>[2x]MHHHHHHSSENLYFQGHMASMRIPEDVRKDIPLTNEVIYFDNTATSLTPKPVVEAMDEYYLKYRANVHRGVHRLSQMATHKYEESRKIVADFIGAKFEEIVFTKNTSESLNLVALGLGHIFKRGDKIVTTPYEHHSDLLPWQRLATKLGLKLEFIEGDDEGNLDLSDAEKKIKGAKLVAVQHVSNALGVIHEVEELGKIAKDEGAIFVVDAAQSAGHMEVNVKKLHADFLAFSGHK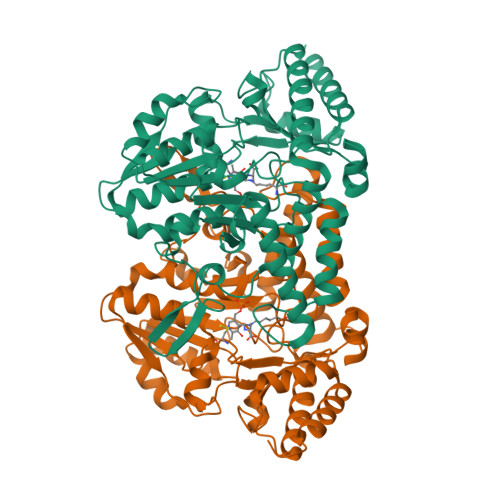GPMGPTGIGVLYIREEFFDTFEPPLIGGGTIEDVSLDGYKLTEPPERFEAGTPNIGGAIGLAAGIRYIERIGLGRIERQEHKLVKRTTEGLDELEVPWYGPRNLKKHAGVVSFNVPGLHPHDVAAILDDHSIMVRSGHHCALPVMKKLGINGTVRASFHVYNSLEEVETFLGVMEELVKGLKT> APLAQQTCANNRHQCSVHA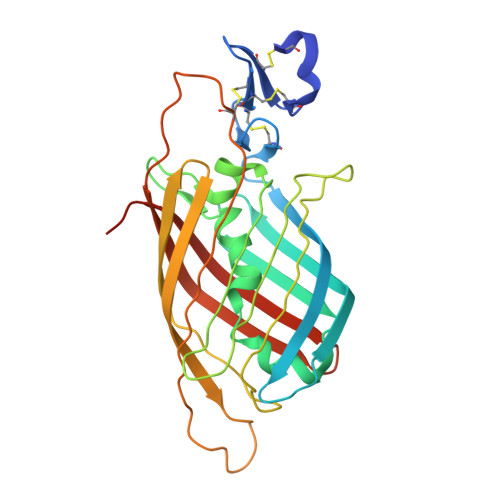ECRDYATGFCCRCVANYTGNGRQCVAEGSPQRVNGKVKGRIFVGSSQVPVVFENTDLHSYVVMNHGRSYTAISTIPETVGYSLLPLAPIGGIIGWMFAVEQDGFKNGFSITGGEFTRQAEVTFLGHPGKLVLKQQFSGIDEHGHLTISTELEGRVPQIPYGASVHIEPYTELYHYSSSVITSSSTREYTVMEPDQDGAAPSHTHIYQWRQTITFQECAHDDARPALPSTQQLSVDSVFVLYNKEERILRYALSNSIGPVRDGSPDA>SNAMEVTVPATLNVLNGSDARLPCTFNSAYTVNHKQFSLNWTYQEANNASEEMFLQFRMKIINLKLERFQDRVEFSGNPSKYDVSVMLRNVQPEDEGIYNCYIMNPPDRHRGHG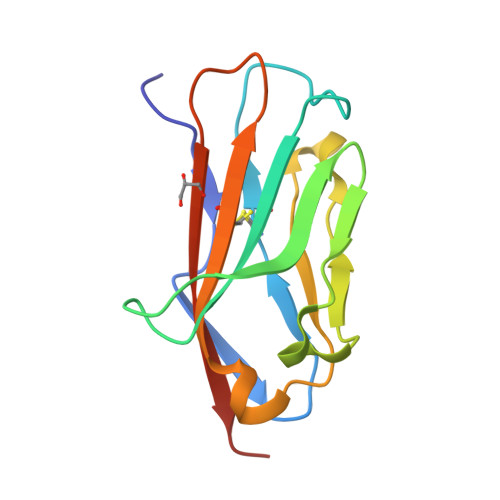KIHLQVLMEEPPE[2x]>GSVLQKEGIEISEGTGYDLSKEPGAATVKALEQGTIVI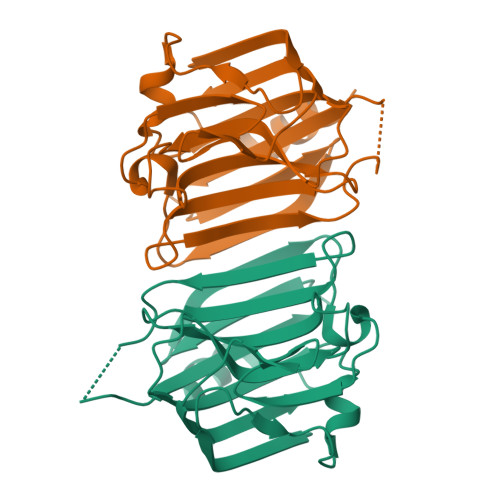SYKTTSENAIQSLLSVGNGTKGNQDRHFHLYITNAGGVGMELRNTDGEFKYTLDCPAAVRGSYKGERVSNTVALKADKENKQYKLFANGELIATLDQEAFKFISDITGVDNVMLGGTMRQGTVAYPFGGSIERMQVYRDVLSDDELIAVTGK[2x]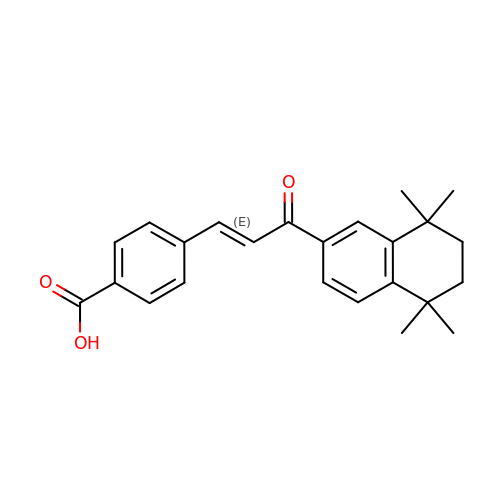4-[3-OXO-3-(5,5,8,8-TETRAMETHYL-5,6,7,8-TETRAHYDRO-NAPHTHALEN-2-YL)-PROPENYL]-BENZOIC ACID | C24 H26 O3 | ZXQHMEUGMCXKLO-KPKJPENVSA-N4-[7-azanyl-8-(7-fluoranyl-1H-indazol-4-yl)-6-oxidanylidene-5H-1,5-naphthyridin-3-yl]-N,N-dimethyl-benzamide | C24 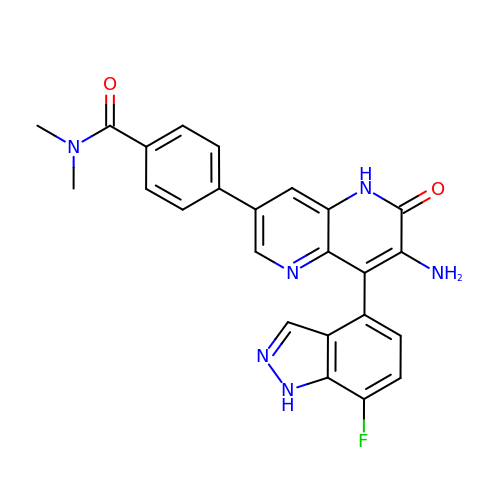H19 F N6 O2 | GQHFJDVSIFLECJ-UHFFFAOYSA-N> GSHMDGTEKWRFKTGKAIEASPVIGEDGTIYVGSNDGHLYAINPDGTEKWRFKTGKAIEASPVIGEDGTIYVGSNDGHLYAINPDGTEKWRFKTGKAIEASPVIGEDGTIYVGSNDGHLYAINPDGTEKWRFKTGKAIEASPVIGEDGTIYVGSNDGHLYAINPDGTEKWRFKTGKAIEASPVIGEDGTIYVGSNDGHLYAINPDGTEKWRFKTGKAIEASPVIGEDGTIYVGSNDGHLYAINPDGTEKWRFKTGKAIEASPVIGEDGTIYVGSNDGHLYAINPDGTEKWRFKTGKAIEASPVIG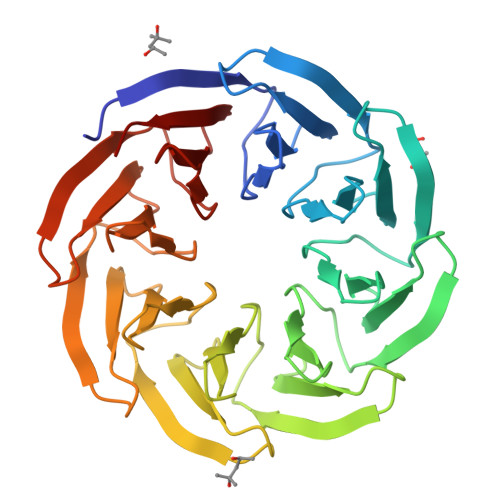EDGTIYVGSNDGHLYAINP> DPDQFRAIIESPEGAGHVGYQYRRNTGSTMRMVSDVLDERVSLWDFHCDPSGNVIQPGPNVDSRQYLQAAIDYVSSNGGGTITIPAGYTWYLGSYGVGGIAGHSGIIQLRSNVNLNIEGRIHLSPFFDLKPFQVFVGFDNGDPASSGNLENCHIYGHGVVDFGGYEFGASSQLRNGVAFGRSYNCSVTGITFQNGDVTWAITLGWNGYGSNCYVRKCRFINLVNSSVNAAHSTVYVNCPYSGVESCYFSMSSSFARNIACSVELHQHDTFYRGSTV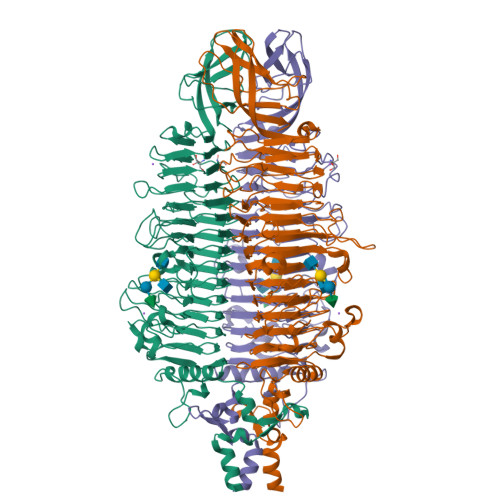NGYCRGAYVVMHAAEAAGAGSYAYNMQVENNIAVIYGQFVILGSDVTATVSGHLNDVIVSGNIVSIGERAAFSAPFGAFIDIGPDNSGASNVQDIQRVLVTGNSFYAPANITDSAAITLRANLNGCTFIANNFDCRYMVYNAPGTTSPVVQNLVWDKSNVIGGTHANQRAGQNLFDMQFASVVNSTIEVQLSCEDLSMFSCILFPASCQLSYSKITVDSAWTKSMSNTAVFEGNQQAGANVYVSYPATVNLTSYNTQGAVPFFSTDTNYAWVTSAYSLSINENLDFSPPATYTNKANGQLVGVGYNEIGGVRSVSVRLMLQRQV Glutathione transferases (GSTs) are a superfamily of proteins found in all cellular organisms, which usually exist as multiple isoforms. One general function of this superfamily is the involvement in detoxication reactions for both endogenous and xenobiotic compounds. In insects, the Delta and Epsilon class GSTs make major contributions to detoxication of insecticides, contributing to insecticide resistance. We report a new Epsilon class protein crystal structure from Drosophila melanogaster for the glutathione transferase DmGSTE6.

In the present study, we have determined the structure of DmGSTE6 to supplement the currently known Epsilon structures. This structure adopts the typically highly conserved GST fold with two domains comprising a βαβαββα motif in the N-terminus and an all α-helical domain in the C-terminus. The Epsilon clasp motif comprises an extended ‘wafer’ arrangement of four histidines (two contributed from each subunit), which is supported by interactions with several conserved serines from helices 3, 4 and 6. His101 from one subunit wraps around the His101 from the other subunit to generate the clasp motif also seen in the Delta GST class. In the Epsilon DmGSTE6, a second histidine in each subunit, His69, interacts with clasp His101 from the other subunit. These His–His interactions are also supported by three serines, Ser68, Ser104, Ser163, in each subunit. Furthermore, Ser68 directly interacts with GSH in the active site as the Ser68 OG and N atoms are within 2.5–3.3 Å of the GSH O11 and O12 atoms. The His69 ND1 atom is also within the interaction distance of 3.5 Å of the GSH O12 atom. The current structure also shows that the active site pocket for Epsilon class GSTs is more in a ‘closed’ configuration than that of Delta class. Arg113 is conserved only in the Epsilon class and it interacts with the glutamyl part of GSH, suggesting that this residue may play a role in modulating GSH/hydrophobic substrate conjugation. From superposition the residues for DmGSTE6 that would generate a hydrophobic binding cavity for HNE appear to be Ser12 (catalytic residue); Pro11, Pro13, Pro14 (N-terminus helix 1); Ile36 (coil between beta strand 2 and helix 2); Phe108, Ile112, Arg113, Leu120 (helix 4); Phe174 (C-terminus helix 7); Leu209, Phe213 (helix 9).

>MVKLTLYGLDPSPPVRAVKLTLAALNLTYEYVNVDIVARAQLSPEYLEKNPQHTVPTLEDDGHYIWDSHAIIAYLVSKYADSDALYPKDPLKRAVVDQRLHFESGVVFANGIRSISKSVLFQGQTKVPKERYDAIIEIYDFVETFLKGQDYIAGNQLTIADFSLVSSVASLEAFVALDTTKYPRIGAWIKKLEQLPYYEEANGKGVRQLVAIFKKTNFTFEA[4x]> MLSRKGIIPEEYVLTRLAEDPTEPRYRTRERRARFVSKKGNCNVAHKNIREQGRFLQDVFTTLVDLKWPHTLLIFTMSFLCSWLLFAMVWWLIAFAHGDLAPGEGTNVPCVTSIHSFSSAFLFSIEVQVTIGFGGRMVTEECPLAILILIVQNIVGLMINAIMLGCIFMKTAQAHRRAETLIFSKHAVITPRHGRLCFMLRVGDLRKSMIISATIHMQVVRKTTSPEGEVVPLHQVDIPMENGVGGNSIFL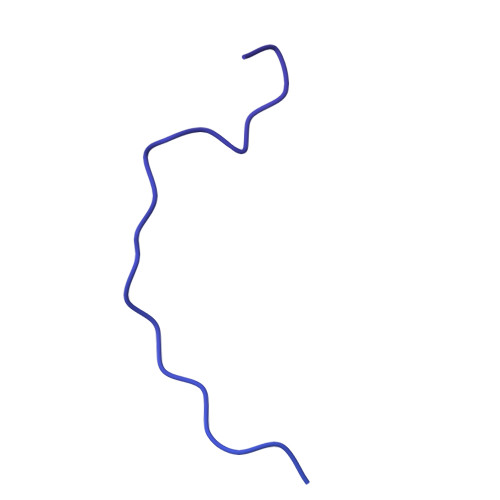VAPLIIYHVIDSNSPLYDLAPSDLHHHQDLEIIVILEGVVETTGITTQARTSYLADEILWGQRFVPIVAEEDGRYSVDYSKFGNTVKVPTPLCTARQLDEDRSLLDALTLASSRGPLRKRSVAVAKAKPKFSISPDSLS>MHHHHHHMIPAECTTIYNRGEHTSGMYAIRPSNSQVFHVYCDVISGSPWTLIQHRIDGSQNFNETWENYKYGFGRLDGEFWLGLEKIYSIVKQSNYVLRIELEDWKDNKHYIEYSFYLGNHETNYTLHLVAITGNVPNAIPENKDLVFSTWDHKAKGHFNCPEGYSGGWWWHDECGENNLNGKYNKP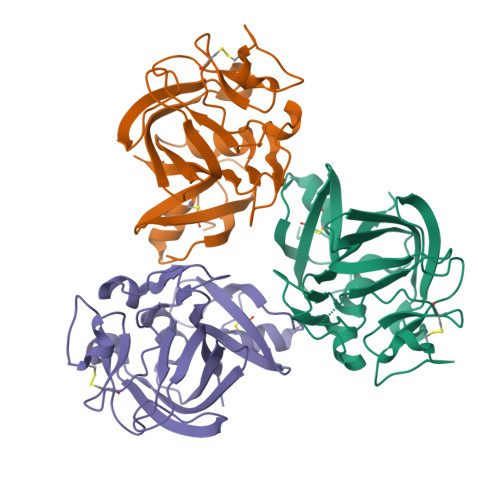RAKSKPERRRGLSWKSQNGRLYSIKSTKMLIHPTDSESFE[3x]>[4x]MDIKINDITLGNNSPFVLFGGINVLESLDSTLQTCAHYVEVTRKLGIPYIFKASFDKPRSSIHSYRGVGLEEGLKIFEKVKAEFGIPVITDVHEPHQCQPVAEVCDVIQLPAFLARQTDLVVAMAKTGNVVNIKKP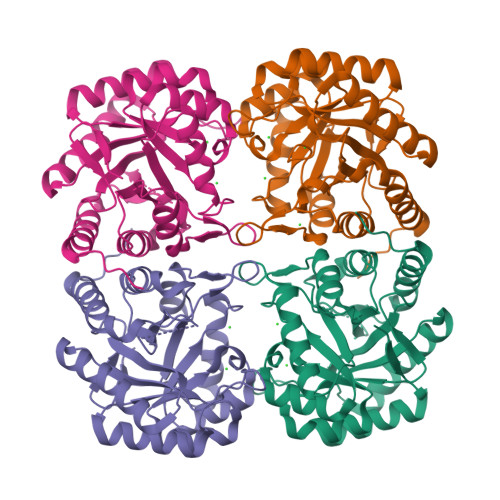QFLSPSQMKNIVEKFHEAGNGKLILCERGSSFGYDNLVVDMLGFGVMKQTCGNLPVIFDVTHSLGRRAQALDLALAGMATRLAGLFLESHPDPKLAKCDGPSALPLHLLEDFLIRIKALDDLIKSQPILTIE3-(benzotriazol-1-yl)-5-[1-methyl-5-[(1~{S})-1-morpholin-4-ylethyl]-1,2,4-triazol-3-yl]pyrazin-2-amine 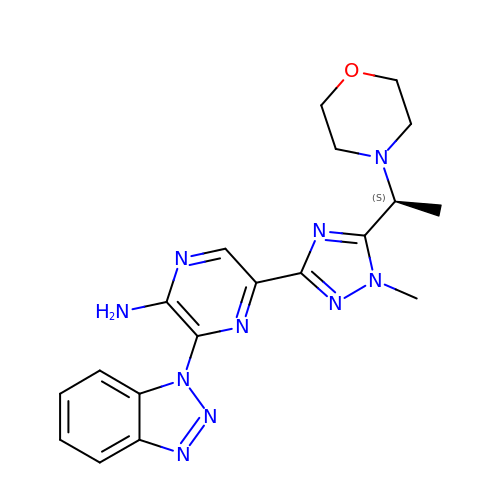| C19 H22 N10 O | FXHVFSHZRDKMCE-LBPRGKRZSA-N>MDITITLDRSEQADYIYQQIYQKLKKEILSRNLLPHSKVPSKRELAENLKVSVNSVNSAYQQLLAEGYLYAIERKGFFVEELDMFSAEEHPPFALPDDLKEIHIDQSDWISFSHMSSDTDHFPIKSWFRCEQKAASRSYRTLGDMSHPQGIYEVRAAITRLISLTRGVKCRPEQMIIGAGTQVLMQLLTELLPKEAVYAMEEPGYRRMYQLLKNAGKQVKTIMLDEKGMSIAEITRQQPDVLVTTPSHQFPSGTIMPVSRRIQLLNWAAEEPRRYIIEDDYDSEFTYDVDSIPALQSLDRFQNVIYMGTFSKSLLPGLRISYMVLPPELLRAYKQRGYDLQTCSSLTQLTLQEFIESGEYQKHIKKMKQHYKEKRERLITALEAEFSGEVTVKGANAGLHFVTEFDTRRTEQDILSHAAG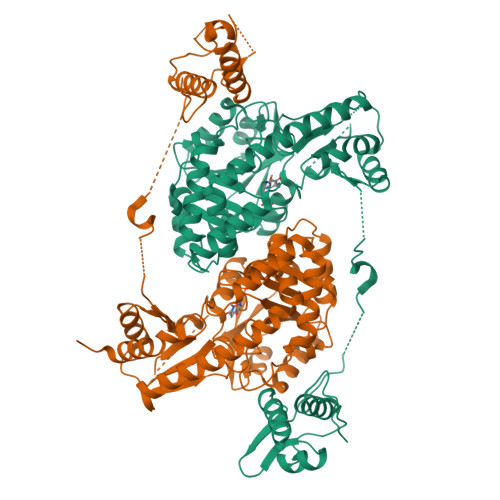LQLEIFGMSRFNLKENKRQTGRPALIIGFARLKEEDIQEGVQRLFKAVYGHKKIPVTGD[4x]N-[3-[(1S,3S,6S)-5-azanyl-3-methyl-4-azabicyclo[4.1.0]hept-4-en-3-yl]-4-fluoranyl-phenyl]-5-chloranyl-pyridine-2-carboxamide 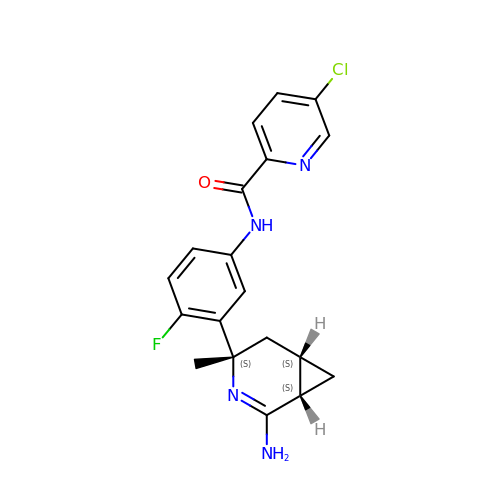| C19 H18 Cl F N4 O | MELPDVINWCDKRF-JXBWDGJFSA-N> VSEIKTLVTFFGGTGDLAKRKLYPSVFNLYKKGYLQKHFAIVGTARQALNDDEFKQLVRDSIKDFTDDQAQAEAFIEHFSYRAHDVTDAASYAVLKEAIEEAADKFDIDGNRIFYMSVAPRFFGTIAKYLKSEGLLADTGYNRLMIEKPFGTSYDTAAELQNDLENAFDDNQLFRIDHYLGKEMVQNIAALRFGNPIFDAAWNKDYIKNVQVTLSEVLGVEERAGYYDTAGALLDMIQNHTMQIVGWLAMEKPESFTDKDIRAAKNAAFNALKIYDEAEVNKYFVRAQYGAGDSADFKPYLEELDVPADSKNNTFIAGELQFDLPRWEGVPFYVRSGKRLAAKQTRVDIVFKAG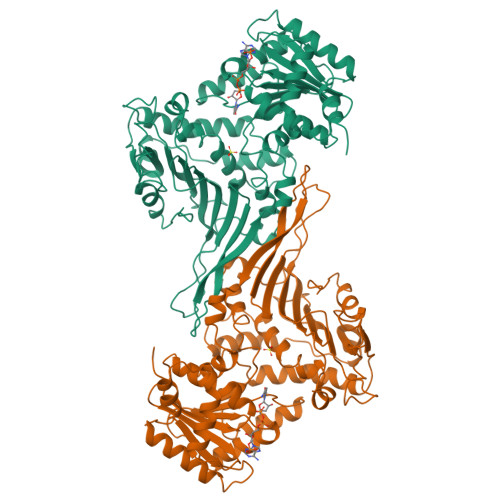TFNFGSEQEACEAVLSIIIDPKGAIELKLNAKSVEDAFNTRTIDLGWTVSDEDKKNTPEPYERMIHDTMNGDGSNFADWNGVSIAWKFVDAISAVYTADKAPLETYKSGSMGPEASDKLLAANGDAWVFKG> MMPVFHTRTIESILEPVAQQIS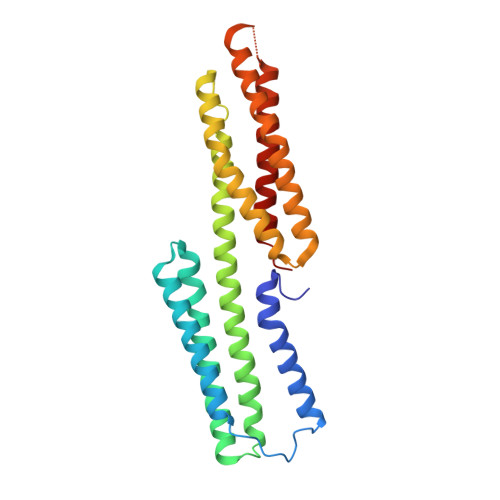HLVIMHEEGEVDGKAIPDLTAPVAAVQAAVSNLVRVGKETVQTTEDQILKRDMPPAFIKVENACTKLVQAAQMLQSDPYSVPARDYLIDGSRGILSGTSDLLLTFDEAEVRKIIRVCKGILEYLTVAEVVETMEDLVTYTKNLGPGMTKMAKMIDERQQELTHQEHRVMLVNSMNTVKELLPVLISAMKIFVTTKNSKNQGIEEALKNRNFTVEKMSAEINEIIRVLQLTS>[3x]AMKNWKTSAESILTTGPVVPVIVVKKLEHAVPMAKALVAGGVRVLNVTLRTECAVDAIRAIAKEVPEAIVGAGTVLNPQQLAEVTE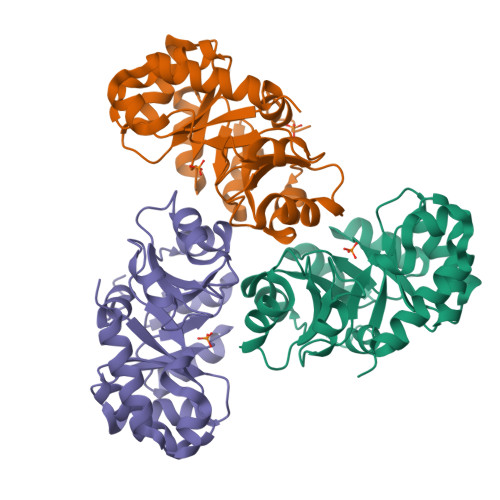AGAQFAISPGLTEPLLKAATEGTIPLIPGISTVSELMLGMDYGLKEFKFFPAEANGGVKALQAIAGPFSQVRFCPTGGISPANYRDYLALKSVLCIGGSWLVPADALEAGDYDRITKLAREAVEGAKL>MRNQDKRAAHKDSEPSTEVNHTASSYQGRQQETGMNLRGIDGNEPTEGSNLLNNNEKMQGTPAEPNHLQRRRQIHACPPRGLLARVITNVTMVILLWAVVWSVTG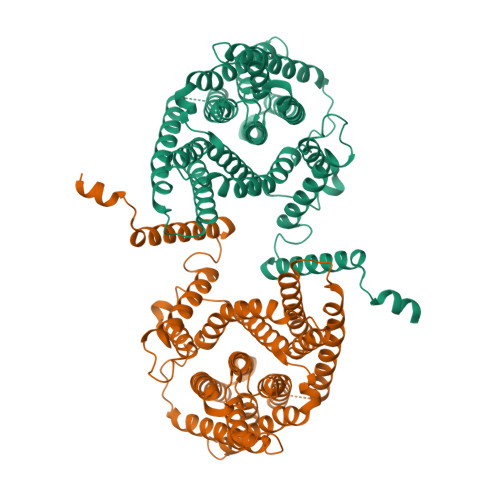SECLPGGNLFGIIMLFYCAIIGGKLFGLIKLPTLPPLPPLLGMLLAGFLIRNVPVISDNIQIKHKWSSALRSIALSVILVRAGLGLDSNALKKLKGVCVRLSLGPCLIEACTSAVLAYFLMGLPWQWGFMLGFVLGAVSPAVVVPSMLLLQEGGYGVEKGIPTLLMAAGSFDDILAITGFNTCLGMAFSTGSTVFNVLKGVLEVIIGVVTGLVLGFFIQYFPSSDQDNLVWKRAFLVLGLSVLAVFSSTYFGFPGSGGLCTLVTAFLAGRGWASTKTDVEKVIAVAWDIFQPLLFGLIGAEVLITALRPETIGLCVATLGIAVLIRILVTYLMVCFAGFNIKEKIFISFAWLPKATVQAAIGSVALDTARSHGEKQLEGYGMDVLTVAFLSIIITAPVGSLLIGLLGPRLLQKAEQNKDEEDQGETSIQV[2x]>[2x]ATFLIWPIYPKIEANEKATAVWLQNTGKTDAMVQIRVFKWNQDGLKDNYSEQSEIIPSPPVAKIKAGEKHMLRLTKSVNLPDGKEQSYRLIVDELPIRLSDGNEQDASKVSFQMRYSIPLFAYGKGIGSGLTEESQKLNAKNALAKPVLQWSVRNNQQGQSELYLKNNGQKFARLSALKTSKTGNDISLGKAAFGYVLSNSTVKFA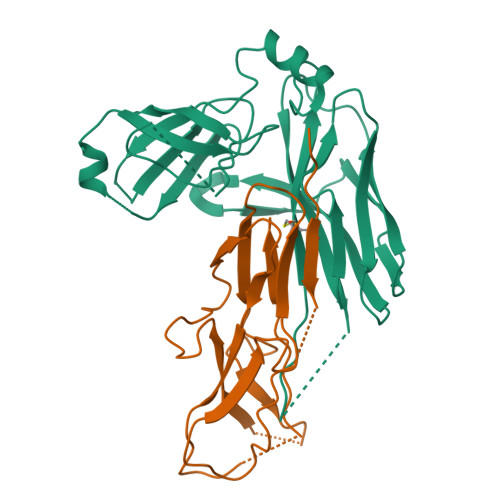IDQSTAHELAKTSKIYGVDSSGIKQELIEITKMEDPS;>AVTHHHHHHSTGCTVGGSQTEGNMNKFGTLNFGKTSGTWNNVLTAEVASAATGGNISVTCDGTDPVDFTVAIDGGERTDRTLKNTASADVVAYNVYRDAARTNLYVVNQPQQFTTVSGQATAVPIFGAIAPNTGTPKAQGDYKDTLLVTVNF[2x]> VILPNNNRHQIFNTTQGHYDAVSFIYIPIDGGYMSGSGVVVGENEILTNKHVVNGAKGNPRNISVHPSAKNENDYPNGKFVGQEII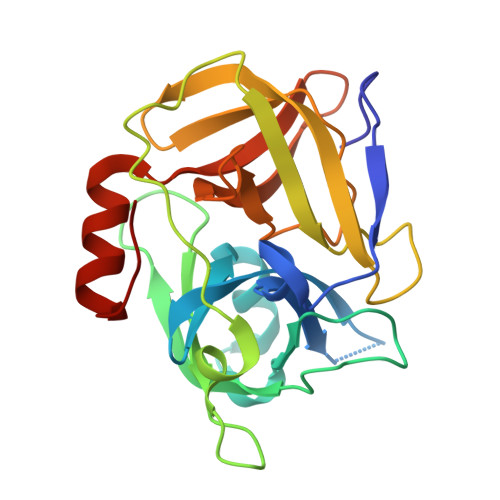PYPGNSDLAILRVSPNEHNQHIGQVVKPATISSNTDTRINENITVTGYPGDKPLATMWESVGKVVYIGGEELRYDLSTVGGNAGSPVFNGKNQVIGIHYGGVDNKYNSSVYINDFVQQFLRNNIPDINIQ4-[(2~{S})-2-carboxy-5-(oxidanylamino)-5-oxidanylidene-pentyl]benzoic acid | C13 H15 N O6 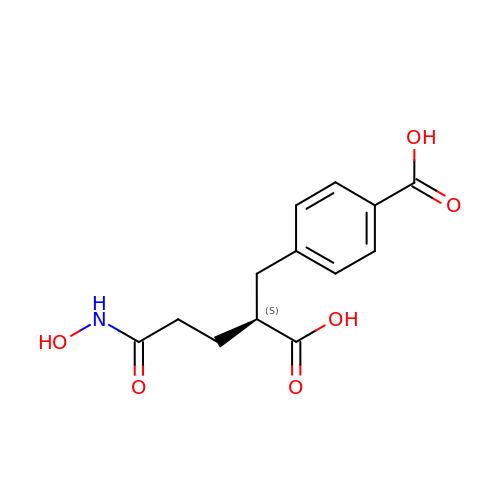| VUDGMYIWOPKVSL-JTQLQIEISA-N> MSVTIDHTTENAAPAQAPVSDRAWALFRALDGKGLVPDGYVEGWKKTFEEDFSPRRGAELVARAWTDPEFRQLLLTDGT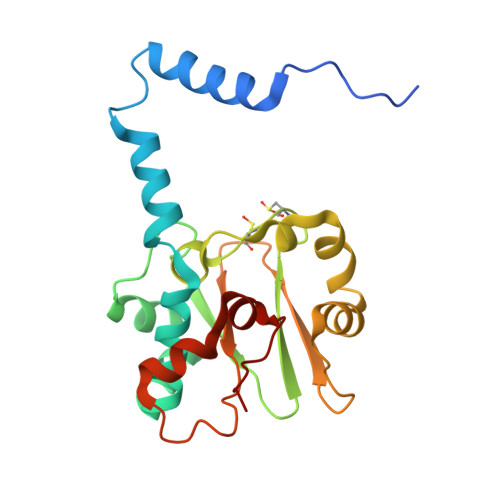AAVAQYGYLGPQGEYIVAVEDTPTLKNVIVCSLCSCTAWPILGLPPTWYKSFEYRARVVREPRKVLSEMGTEIASDIEIRVYDTTAETRYMVLPQRPAGTEGWSQEQLQEIVTKDCLIGVAIPQVPTV> MPKPINVRVTTMDAELEFAIQPNTTGKQLFDQVVKTVGLREVWFFGLQYVDSKGYSTWLKLNKKVTQQDVKKENPLQFKFRAKFFPEDVSEELIQEITQRLFFLQVKEAILNDEIYCPPETAVLLASYAVQAKYGDYNKEIHKPGYLANDRLLPQRVLEQHKLTKEQWEERIQNWHEEHRGMLREDSMMEYLKIAQDLE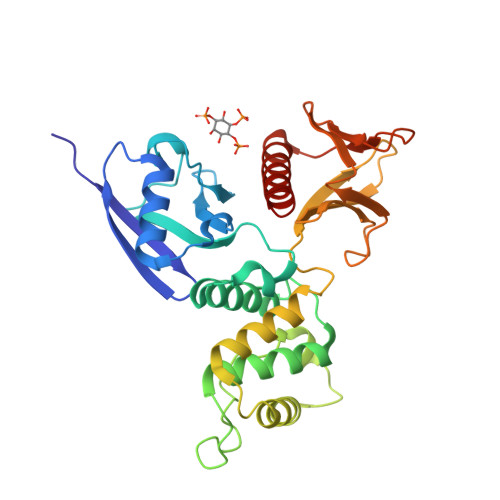MYGVNYFEIKNKKGTELWLGVDALGLNIYEHDDKLTPKIGFPWSEIRNISFNDKKFVIKPIDKKAPDFVFYAPRLRINKRILALCMGNHELYMRRRKP> MGSSHHHHHHSSGLVPRGSHMAGERVSDTPTQRDPVFEILQSRGRRSPAVWFHGSMGTVQAYLGLARAIGDEVPFHAFQSRGLRGEDAPLADLGEMAALYTR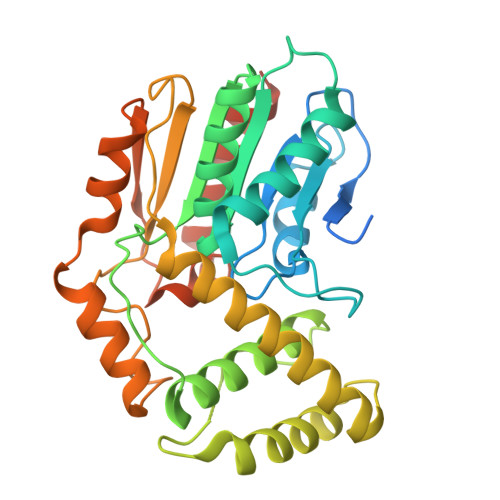RLLARQPDESRAFRLGGYSQGGLLAYEVTRQLQLAGRRVESLVMVDTPYAYGDMALKDDDDTDSLRLAIVYVNLLLMNGLGDFSDLAEVHRPGIDPAELLPALVRAGIDRGLPYTPQALGQLIERHHRVARANETAARTYLPADLPHPGQPVVHYFARRHPQVYFDPARFSGPMVEWTNRYFADKDCASRWQRHLPTWHHHATPAVDHFAMLTDSASFAAIVRTCRELYLGSGSTTDQAGALLVSGPA> SMTEEERSSALSEVSLRLLCHDDIDTVKHLCGDWFPIEYPDSWYRDITSNKKFFSLAATYRGAIVGMIVAEIKNRTKIHKEDGDILASNFSVDTQVAYILSLGVVKEFRKHGIGSLLLESLKDHISTTAQDHCKAIYLHVLTTNNTAINFYENRDFKQHHYLPYYYSIRGVLKDGFTYVLYINGGHPPWTILDYIQHLGSALASLSPCSIPHRVYRQAHSLLCSFLPWSGISSKSGIEYSRTM

As the first N-terminal acetyltransferase discovered on an organelle, NatF, encoded by NAA60 and also named as Histone acetyltransferase type B protein 4 (HAT4), Naa60 or N-acetyltransferase 15 (NAT15), is the youngest member of the NAT family. As an N-terminal acetyltransferase, NatF can specifically catalyze acetylation of the N-terminal α-amine of most transmembrane proteins and has substrate preference towards proteins with Met-Lys-, Met-Val-, Met-Ala- and Met-Met-N-termini, thus partially overlapping substrate selectivity with NatC and NatE18. Another important feature of NatF is that this protein is anchored on the Golgi apparatus through its C-terminal membrane-integrating region and takes part in the maintaining of Golgi integrity. The structure of hNaa60 protein contains a central domain exhibiting a classic GCN5-related N-acetyltransferase (GNAT) folding, along with the extended N- and C-terminal regions.

There is one hNaa60 molecule in the asymmetric unit in the hNaa60(1-242)/Ac-CoA structure. The C-terminal region extended from the GCN5-domain forms an amphipathic helix (α5) and interacts with a molecule in a neighbor asymmetric unit through hydrophobic interactions between α5-helix and a hydrophobic groove between the N-terminal β1 and β3 strands of the neighbor molecule. In hNaa60(1-242), the β7-β8 hairpin is located in close proximity to the α1-α2 loop, creating a more compact substrate binding site than that in hNaa50, where this region adopts a more flexible loop conformation (β6-β7 loop). In hNaa60(1-242), the β7-β8 hairpin covers the active site in a way similar to that observed in hNaa50, presumably leaving only one way for the substrate to access the active site, i.e. to enter from the opposite end into the same tunnel where Ac-CoA/CoA binds, which may accommodate access of a NAT substrate only. Indeed, superposition of hNaa60(1-242) structure on that of Hat1p, a typical KAT, in complex with a histone H4 peptide27 revealed obvious overlapping/clashing of the H4 peptide (a KAT substrate) with the β7-β8 hairpin of hNaa60(1-242). A solvent-derived malonate molecule is found beside Phe 34 and the ethanethioate moiety of Ac-CoA in the high-resolution hNaa60(1-242)/Ac-CoA structure. Superposition of this structure on that of hNaa50p/CoA/peptide shows that the malonate molecule overlaps well on the N-terminal methionine of the substrate peptide and residue Phe 34 in hNaa60 overlaps well on Phe 27 in hNaa50. However, in the hNaa60/Ac-CoA structure, a hydrophilic malonate molecule is found at the same location where the N-terminal methionine should bind as is indicated by the superposition, suggesting that Phe 34 may accommodate binding of hydrophilic substrate, too. Residues Tyr 38, Asn 143 and Tyr 165 are located around the malonate and interact with it through direct hydrogen bonds or water bridge.5-bromanyl-2-(5,6,7,8-tetrahydronaphthalen-2-ylsulfonylamino)benzoic 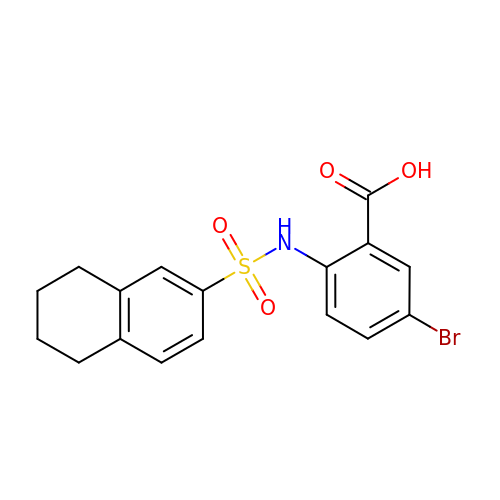acid | C17 H16 Br N O4 S | PCBPZTPLEQENRQ-UHFFFAOYSA-N>MSSASSNARDEVIAAIHEEADWVDRTVYPFESRCIGLSSGAVHYIDEGPDDGGRETLLMLHGNPTWSFLYRHLVRDLRDEYRCVALDYLGFGLSERPTDFSYRPEDHADVVEEFIDELGLEDVVLVGHDWGGPIGFSYAIDHPENVGGLVVMNTWMWPVSDDKHFSRFSKLLGGRIGRELCERYDLFTRVIMPMGFADRSRFTESAREQYRAANRGDRTGTGIFPQAILGSRAWLSSLWEQRDNIADIPARIIWGMEDSAFRPAELRTFEALFEDSSTVRLYGVGHYVPEEFGSDLVPLVREFLEEVLEVLFQ[2x]

Haloalkane dehalogenases (EC 3.8.1.5, HLDs) are a group of enzymes that catalyze the hydrolytic cleavage of a carbon–halogen bond in a range of halogenated organic compounds. Here we probe the structural organization of DhmeA, a subfamily III HLD‐like enzyme from the archaeon Haloferax mediterranei, by combining cryo‐electron microscopy (cryo‐EM) and x‐ray crystallography. A distinct catalytic pentad forms the active site of HLD enzymes: a nucleophile aspartic acid, a histidine base, a catalytic acid (aspartic or glutamic acid) and two halide stabilizing residues (two tryptophans or tryptophan + asparagine) (Janssen, 2004). We show that full‐length wild‐type DhmeA forms diverse quaternary structures, ranging from small oligomers to large supramolecular ring‐like assemblies of various sizes and symmetries.

The cryo‐EM data collected on optimized DhmeA sample showed particles with tentative threefold symmetry. Therefore, we have used a strategy addressing the issue of non‐uniform particle orientation distribution by combining data collected at different sample tilt (Tan et al., 2017). The cryo‐EM map reconstructed from the major class of the particles present in the data showed six DhmeA molecules arranged into a D3 assembly. The resolution of the final model was limited to 7–8 Å which limited further data analysis. We have tested both focused refinement and focused classification of a single DhmeA cryo‐EM density. None of the focused data refinement strategies led to improvement of model resolution which suggests that wild‐type DhmeA forms a highly dynamic assembly. No individual secondary structure elements were clearly defined in the cryo‐EM map, with the exception of a central eight‐stranded β‐sheet that could be unambiguously located. The structure is built from three DhmeA dimers, which are arranged around a 3‐fold symmetry axis. The dimerization interface seems to be tightly packed, while inter‐dimer contacts are less tight. We therefore deduce that the dimeric unit is a common building block of large assemblies formed by wild‐type DhmeA.~{N}-[[4,4-bis(fluoranyl)-1-oxidanyl-cyclohexyl]methyl]-6-fluoranyl-4-oxidanylidene-chromene-2-carboxamide 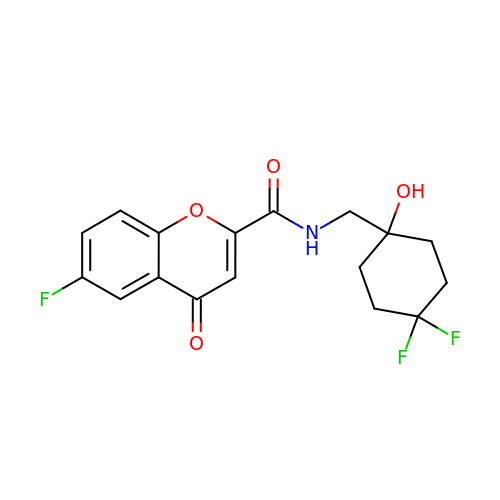| C17 H16 F3 N O4 | PJBRCGHQNUWERQ-UHFFFAOYSA-N Muramidases are N-acetylmuramide glycanhydrolases which cleave the β-1,4-glycosidic bond between N-acetylmuramic acid (NAM) and N-acetylglucosamine (NAG) in the carbohydrate backbone of the bacterial cell-wall peptidoglycan. Here, the identification, characterization and X-ray structure of a novel fungal GH24 muramidase from Trichophaea saccata is first described, in which an SH3-like cell-wall-binding domain (CWBD) was identified by structure comparison in addition to its catalytic domain. A ‘domain-walking’ approach, searching for other sequences with a domain of unknown function appended to the CWBD, was then used to identify a group of fungal muramidases that also contain homologous SH3-like cell-wall-binding modules, the catalytic domains of which define a new GH family. The properties of some representative members of this family are described as well as X-ray structures of the independent catalytic and SH3-like domains of the Kionochaeta sp., Thermothielavioides terrestris and Penicillium virgatum enzymes.

Further, a complex between a triglycine peptide and the CWBD from T. saccata is presented that shows a possible anchor point of the peptidoglycan on the CWBD. However, they are conserved in all examples that we have identified of this CWBD. Structure comparisons using GESAMT revealed a similarity to SH3 domains as mentioned in Section 1. The peptide in the TsGH24 fungal muramidase SH3-like domain is bound on a different face of the molecule to that in the lysostaphin complex, which is in agreement with the discussion in the lysostaphin study: the peptides in bacterial SH3b domains are found in a location remote from the canonical specificity zone of the eukaryotic proteins. The triglycine in our structure is bound within the canonical specificity zone. A thermal shift assay using differential scanning by the fluorimetry (nanoDSF) method was used to confirm that the interaction with triglycine is genuine rather than mediated by zinc ions. The results show that at pH 8.5, which is the pH of the crystallization conditions, the thermal shift is present for both treated and untreated samples, implying ligand binding. However, the CWBD–triglycine structure demonstrates that a peptide ligand can be bound to this SH3 domain and it is located within the specificity zone. The structure of the complex with triglycine provided an additional argument in favour of these domains binding peptide bridges in peptidoglycan, similar to what was observed for the SH3b domains of lysostaphin, which Staphylococcus capitis and S. simulans use in their competition with the other staphylococci.

>[2x]YPVKTDLHCRSSPSTSASIVRTYSSGTEVQIQCQTTGTSVQGSNVWDKTQHGCYVADYYVKTGHSGIFTTKCGS;>[2x]GGG> MAKVEQVLSLEPQHELKFRGPFTDVVTTNLKLGNPTDRNVCFKVKTTVPRRYCVRPNSGVIDAGASLNVSVMLQPFDYDPNEKSKHKFMVQS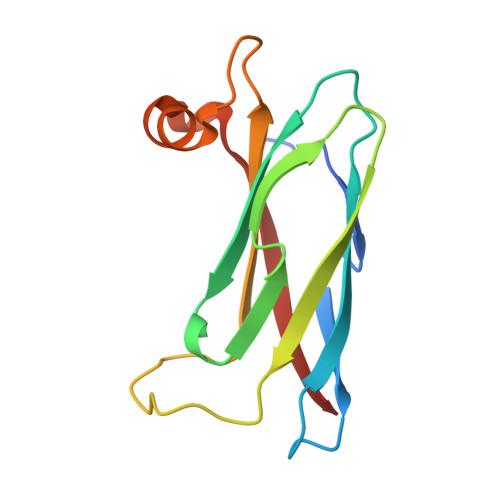MFAPPDTSDMEAVWKEAKPEDLMDSKLRCVFEL> MQPPVANFCLWNLQPIQGSWMGAACIYQMPPSVRNTWWFPLLNTIPLDQYTRIYQWFMGVDRDRSGTLEINELMMGQFPGGIRLSPQTALRMMRIFDTDFNGHISFYEFMAMYKFMELAYNLFVMNDRNRSGTLEPHEILPALQQLGFYINQRTSLLLHRLFARGMAFCDLNCWIAICAFAAQTRSAYQ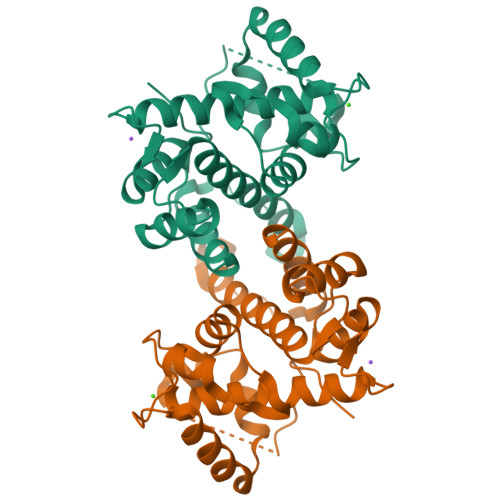MIFMNPYYGPMKPFNPMEFGKFLDVVTSLLE OmCI is a bifunctional protein derived from blood-feeding ticks that specifically prevents complement (C)-mediated C5 activation and also sequesters leukotriene B4 (LTB4) within an internal binding pocket. The 17-kDa lipocalin Ornithodoros moubata complement inhibitor OmCI, originally isolated from an ectoparasitic tick (Acari), is a bifunctional protein that may have such therapeutic advantages. By binding directly to C5 in the vicinity of the C5-C345C domain OmCI prevents cleavage of C5 by the C5 complement convertases, thereby preventing release of anaphylatoxin C5a and formation of the terminal 5b-9 C complex (TCC). We describe two crystal structures of bacterially expressed OmCI: one binding a C16 fatty acid and the other binding LTB4 (C20).

cis-palmitoleic acid (C16H30O2) was the dominant (∼64%) fatty acid in the binding pocket of bOmCI, with various other C16–C18 linear fatty acids present in lower proportions. All ligands fit into the L-shaped pocket, with the kink at position C12 of LTB4, ricinoleic acid, and palmitoleic acid. Palmitoleic acid lacks the -OH group at this position, and in that complex the same OmCI residues coordinate a water molecule instead. The ligands are also of different lengths (C16, C18, and C20, respectively, for palmitoleic acid, ricinoleic acid, and LTB4); LTB4 fills the pocket completely, whereas the yOmCI-ricinoleic acid and bOmCI-palmitoleic acid complexes show a water molecule filling the bottom of the pocket. The three ligands all bind with their carboxylic acid head at the solvent-exposed brim of the OmCI pocket, hydrogen bonding to the side chains of Arg-54, Thr-85, and Trp-87. The hydrophobic side chains of Phe-36, Tyr-43, Leu-57, Gly-59, Pro-61, Leu-70, Val-72, Met-74, Phe-76, Trp-87, Phe-89, Arg-107, and Trp-133 contact the hydrophobic body of all three ligands. The main ligand-dependent structural difference with respect to the yOmCI-ricinoleic acid crystal structure is the position of the loop βB-βC (residues 61–70), which pushes in/out to accommodate a smaller/larger ligand. This movement is mediated by Pro-61, the residue at the bottom of the ligand pocket. The other main locus of structural variability in the bOmCI and yOmCI structures is the conformation of the βH-α3 loop (amino acids 132–142), shown previously to be required for C5 inhibition, which in both complexes of bOmCI swings inward, with the concomitant flip of the side chain of His-117. However, the chemical nature of the ligand in the pocket bears no relationship to the conformation of the βH-α3 loop, as the loop was observed in both conformations in different copies of the yOmCI-ricinoleic acid complex.

> DSESDCTGSEPVDAFQAFSEGKEAYVLVRSTDPKARDCLKGEPAGEKQDNTLPVMMTFKNGTDWASTDWTFTLDGAKVTATLGNLTQNREVVYDSQSHHCHVDKVEKEVPDYEMWMLDAGGLEVEVECCRQKLEELASGRNQMYPHLKDC> GVGISTGTFNNQTEFKFLENGWVEITANSSRLVHLNMPESENYRRVVVNNMDKTAVNGNMALDDIHAQIVTPWSLVDANAWGVWFNPGDWQLIVNTMSELHLVSFEQEIFNVVLKTVSESATQPPTKVYNNDLTASLMVALDSNNTMPFTPAAMRSETLGFYPWKPTIPTPWRYYFQWDRTLIPSHTGTSGTPTNIYHGTDPDDVQFYTIENSVPVHLLRTGDEFATGTFFFDCKPCRLTHTWQTNRALGLPPFLNSLPQSEGATNFGDIGVQQDKRRGVTQMGNTNYITEATIMRPAEVGYSAPYYSFEASTQGPFKTPIAAGRGGAQTDENQAADGNPRY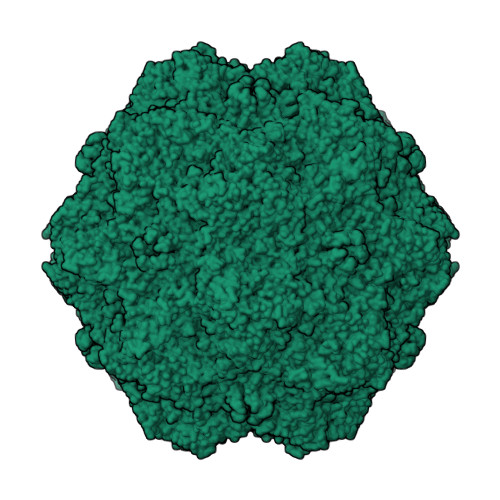AFGRQHGQKTTTTGETPERFTYIAHQDTGRYPEGDWIQNINFNLPVTNDNVLLPTDPIGGKTGINYTNIFNTYGPLTALNNVPPVYPNGQIWDKEFDTDLKPRLHVNAPFVCQNNCPGQLFVKVAPNLTNEYDPDASANMSRIVTYSDFWWKGKLVFKAKLRASHTWNPIQQMSINVDNQFNYVPSNIGGMKIVYEKSQLAPRKLY> GAMDSSEMSTICDKTLNPSFCLKFLNTKFASANLQALAKTTLDSTQARATQTLKKLQSIIDGGVDPRSKLAYRSCVDEYESAIGNLEEA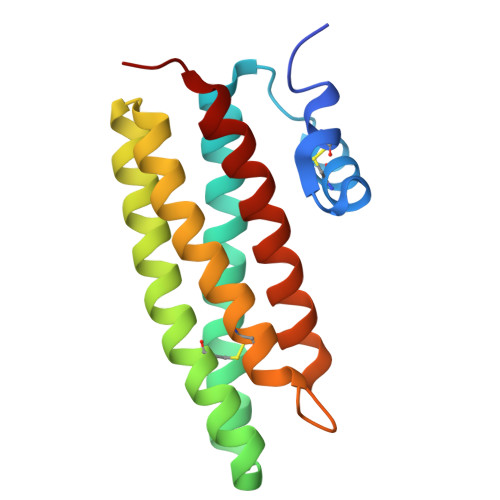FEHLASGDGMGMNMKVSAALDGADTCLDDVKRLRSVDSSVVNNSKTIKNLCGIALVISNMLPRN> MHHHHHHITSLYKKAGFMKGIYSALMVPYN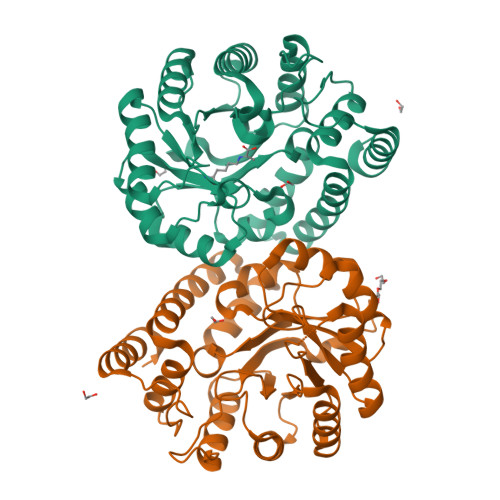EDGSINEKGLREIIRYNIDKMKVDGLYVGGSTGENFMISTEEKKRVFEIAIDEAKDSVNLIAQVGSINLNEAVELGKYVTKLGYKCLSAVTPFYYKFDFSEIKDYYETIVRETGNYMIIYSIPFLTGVNMSLSQFGELFENEKIIGVKFTAGDFYLLERVRKAFPDKLIFAGFDEMLLPATVLGVDGAIGSTYNINGIRAKQIFELAKNSKIDEALKIQHTTNDLIEGILSNGLYQTIKEILKLEGVDAGYCRKPMKKISQKQIEFAKELHKKFLKN;> LYKKAGFMKGIYSALMVPYNEDGSINEKGLREIIRYNIDKMKVDGLYVGGSTGENFMISTEEKKRVFEIAIDEAKDSVNLIAQVGSINLNEAVELGKYVTKLGYKCLSAVTPFYYKFDFSEIKDYYETIVRETGNYMIIYSIPFLTGVNMSLSQFGELFENEKIIGVKFTAGDFYLLERVRKAFPDKLIFAGFDEMLLPATVLGVDGAIGSTYNINGIRAKQIFELAKNSKIDEALKIQHTTNDLIEGILSNGLYQTIKEILKLEGVDAGYCRKPMKKISQKQIEFAKELHKKFLK Fluorescent proteins have facilitated major breakthroughs in modern molecular cell biology. They are widely used for studying biological events, such as cellular trafficking and endocytosis, and have contributed to the development of innovations such as multiphoton microscopy, genetically-encoded sensors, and super-resolution microscopy. mKate, a derivative of eqFP578 from Entacmaea quadricolor, is a bright, monomeric, far-red fluorescent protein with excitation and emission peaks at 588 nm and 635 nm, respectively. Structural characterization of mKate under different conditions revealed the pH-dependent trans-cis isomerization of its chromophore, a discovery that further aided the development of mKate variants with enhanced optical properties. Using a structure-informed approach, we introduced a minimal set of two mutations in the chromophore environment of mKate. The first mutation, S158A, has been shown to destabilize the trans conformation of the chromophore, whereas the second mutation, S143C, was intended to impact the cis conformation.

Similar to the parent protein mKate, GmKate barely fluoresces at low pH (pH 2.0–4.0). The crystal structure of the dim state (pH 4.0, determined at 2.0 Å resolution) revealed equal occupancy of the trans- and cis-conformations, suggesting that the apparent pKa of cis-trans isomerization is close to 4.0. The trans-conformation is presumably a neutral (protonated) state, since the absorbance maximum remains unchanged at 445 nm in low pH buffers. The loss of fluorescence may be attributed to the non-planar nature of the trans-conformation. For GmKate, pKaPT was determined to be 9.5±0.4, by fitting the 598 nm-absorbance pH titration profile with a first-order Hill equation. pKaTC was roughly estimated to be close to 4.0 based on the crystallographic data at pH 4.0. In the crystal structures of the double-mutant, both cis and trans conformation are present to varying degrees, suggesting that while these two residues in mKate are involved in stabilizing the cis and trans state, they are not required for the isomerization.

>[8x]AAASMSALITENMHMKLYMEGTVNNHHFKCTSEGEGKPYEGTQTMRIKVVEGGPLPFAFDILATSFMYGSKTFINHTQGIPDFFKQSFPEGFTWERVTTYEDGGVLTATQDTSLQDGCLIYNVKIRGVNFPSNGPVMQKKTLGWEACTEMLYPADGGLEGRADMALKLVGGGHLICNLKTTYRSKKPAKNLKMPGVYYVDRRLERIKEADKETYVEQHEVAVARYCDLPSKLAHK> AIDEIKSRGYLLVGLSADFPPFEFVDENGNIVAFDVDLAKEIARRLGVELKIVDMTFDGLIPSLLTKKIDVIISGMTITEERKKVVAFSDPYFD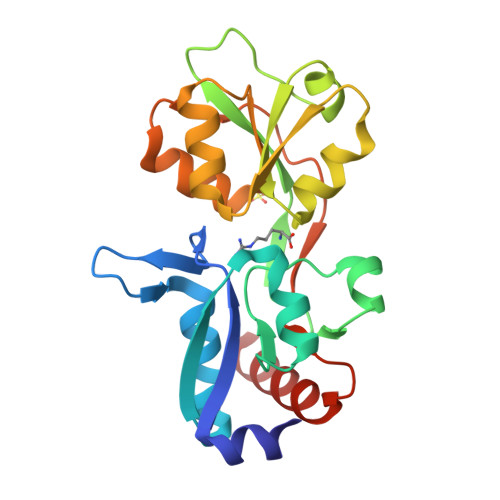AGQVIVVRKDSDFRPKTYEDLVGKTVAVQIGTTGDIEVSKYDGIKVVRFDKFTDAFLELKRGRADAVVLDSATARAFVAKNPDLVISSGVLSSEQYGIAVRKEDTDLLEFINSVLRELK> GLGDELEEVIVEKTKQTVASISSGPKHTQKVPILTANETGATMPVLPSDSIETRTTYMHFNGSETDVECFLGRAACVHVTEIQNKDATGIDNHREAKLFNDWKINLSSLVQLRKKLELFTYVRFDSEYTILATASQPDSANYSSNLVVQAMYVPPGAPNPKEWDDYTWQSASNPSVFFKVGDTSRF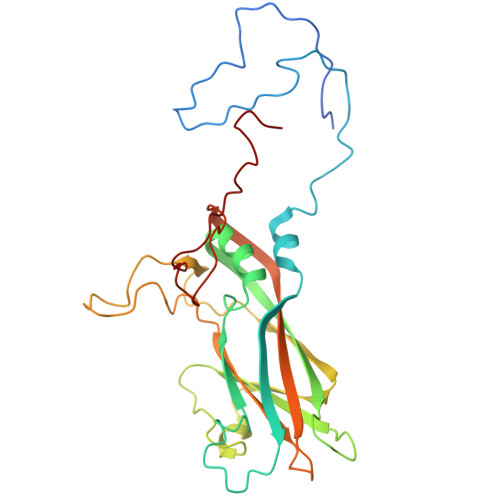SVPYVGLASAYNCFYDGYSHDDAETQYGITVLNHMGSMAFRIVNEHDEHKTLVKIRVYHRAKHVEAWIPRAPRALPYTSIGRTNYPKNTEPVIKKRKGDIKSY> MTTTMKISIEFLEPFRMTKWQESTRRNKNNKEFVRGQAFARWHRNKKDNTKGRPYITGTLLRSAVIRSAENLLTLSDGKISEKTCCPGKFDTEDKDRLLQLRQRSTLRWTDKNPCP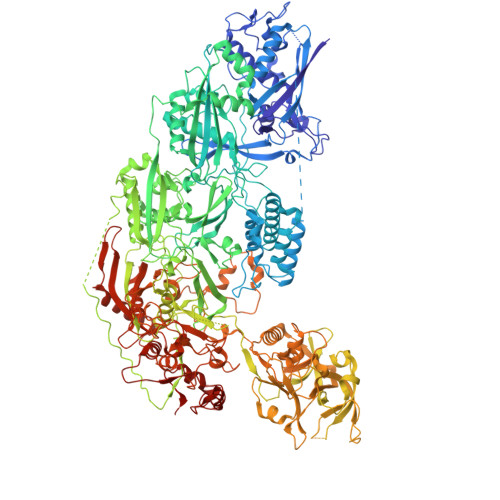DNAETYCPFCELLGRSGNDGKKAEKKDWRFRIHFGNLSLPGKPDFDGPKAIGSQRVLNRVDFKSGKAHDFFKAYEVDHTRFPRFEGEITIDNKVSAEARKLLCDSLKFTDRLCGALCVIRFDEYTPAADSGKQTENVQAEPNANLAEKTAEQIISILDDNKKTEYTRLLADAIRSLRRSSKLVAGLPKDHDGKDDHYLWDIGKKKKDENSVTIRQILTTSADTKELKNAGKWREFCEKLGEALYLKSKDMSGGLKITRRILGDAEFHGKPDRLEKSRSVSIGSVLKETVVCGELVAKTPFFFGAIDEDAKQTDLQVLLTPDNKYRLPRSAVRGILRRDLQTYFDSPCNAELGGRPCMCKTCRIMRGITVMDARSEYNAPPEIRHRTRINPFTGTVAEGALFNMEVAPEGIVFPFQLRYRGSEDGLPDALKTVLKWWAEGQAFMSGAASTGKGRFRMENAKYETLDLSDENQRNDYLKNWGWRDEKGLEELKKRLNSGLPEPGNYRDPKWHEINVSIEMASPFINGDPIRAAVDKRGTDVVTFVKYKAEGEEAKPVCAYKAESFRGVIRSAVARIHMEDGVPLTELTHSDCECLLCQIFGSEYEAGKIRFEDLVFESDPEPVTFDHVAIDRFTGGAADKKKFDDSPLPGSPARPLMLKGSFWIRRDVLEDEEYCKALGKALADVNNGLYPLGGKSAIGYGQVKSLGIKGDDKRISRLMNPAFDETDVAVPEKPKTDAEVRIEAEKVYYPHYFVEPHKKVEREEKPCGHQKFHEGRLTGKIRCKLITKTPLIVPDTSNDDFFRPADKEARKEKDEYHKSYAFFRLHKQIMIPGSELRGMVSSVYETVTNSCFRIFDETKRLSWRMDADHQNVLQDFLPGRVTADGKHIQKFSETARVPFYDKTQKHFDILDEQEIAGEKPVRMWVKRFIKRLSLVDPAKHPQKKQDNKWKRRKEGIATFIEQKNGSYYFNVVTNNGCTSFHLWHKPDNFDQEKLEGIQNGEKLDCWVRDSRYQKAFQEIPENDPDGWECKEGYLHVVGPSKVEFSDKKGDVINNFQGTLPSVPNDWKTIRTNDFKNRKRKNEPVFCCEDDKGNYYTMAKYCETFFFDLKENEEYEIPEKARIKYKELLRVYNNNPQAVPESVFQSRVARENVEKLKSGDLVYFKHNEKYVEDIVPVRISRTVDDRMIGKRMSADLRPCHGDWVEDGDLSALNAYPEKRLLLRHPKGLCPACRLFGTGSYKGRVRFGFASLENDPEWLIPGKNPGDPFHGGPVMLSLLERPRPTWSIPGSDNKFKVPGRKFYVHHHAWKTIKDGNHPTTGKAIEQSPNNRTVEALAGGNSFSFEIAFENLKEWELGLLIHSLQLEKGLAHKLGMAKSMGFGSVEIDVESVRLRKDWKQWRNGNSEIPNWLGKGFAKLKEWFRDELDFIENLKKLLWFPEGDQAPRVCYPMLRKKDDPNGNSGYEELKDGEFKKEDRQKKLTTPWTPWASSGLVPRGSHHHHHH> MDPQGDAAQKTDTSHHDQDHPTFNKITPNLAEFAFSLYRQLAHQSNSTNIFFSPVSIATAFAMLSLGTKADTHDEILEGLNFNLTEIPEAQIHEGFQELLRTLNQPDSQLQLTTGNGLFLSEGLKLVDKFLEDVKKLYHSEAFTVNFGDTEEAKKQINDYVEKGTQGKIVDLVKELDRDTVFALVNYIFFKGKWERPFEVKDTEEEDFHVDQVTTVKVPMMKRLGMFNIQHCKKLSSWVLLMKYLGNATAIFFLPDEGKLQHLENELTHDIITKFLENEDRRSASLHLPKLSITGTYDLKSVLGQL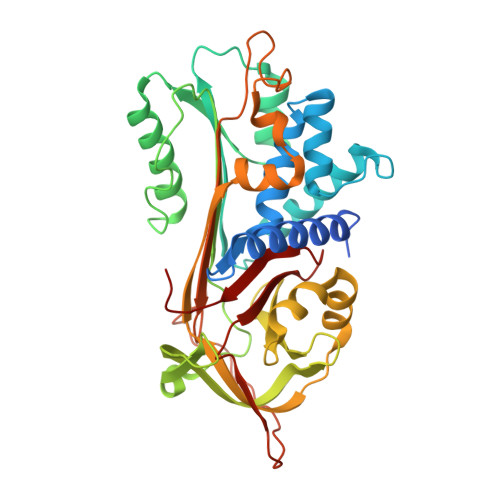GITKVFSNGADLSGVTEEAPLKLSKAVHKAVLTIDEKGTEAAGAMFLEAIPMSIPPEVKFNKPFVFLMIEQNTKSPLFMGKVVNPTQK> GPNDNLEAELEQTKALCEVAKQL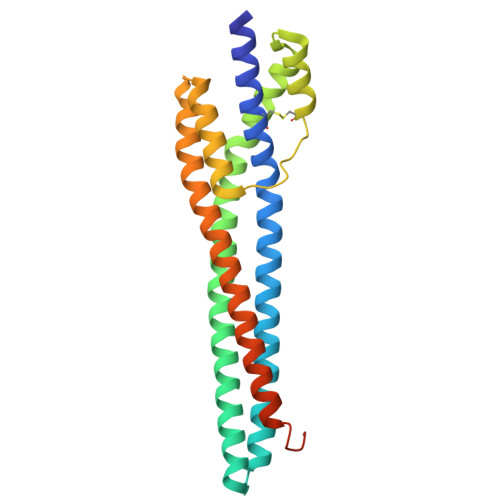RKLPLLTEERRFEAVGALEESKKAAKEGKKAAKRAEAGAVGGTSEQQQAAKRAREAATVAYEASVRAEAAAMEVKRFARALDSFESEYESVFSGLLRGAAEHGGNETIKQLAKECATAVADDVTPEALTRAAHNLRGLYMQDFAEEYLQEANEAANKLEELQKATAETVRAADAADDAKSEAQEEAAQFPEIDDDDSDEDKEDEAS Deeply knotted proteins, whose topologies may introduce substantial barriers to folding, thus represent an interesting test case for protein design. Here we report our attempts to design proteins with trefoil and pentafoil knotted topologies. We extended previously described algorithms for tandem repeat protein design in order to construct deeply knotted backbones and matching designed repeat sequences (N = 3 repeats for the trefoil and N = 5 for the pentafoil). We developed an approach for designing tandem repeat proteins that fold into a class of knotted topologies known as torus knots.

While kcTRP3c.1 and 3c.2 remained recalcitrant to crystallization, crystals of kcTRP3d.1, 3d.2, and 3d.3 grew readily, and their structures were solved via molecular replacement. kcTRP3d.1 and 3d.3 were phased with the original designed atomic coordinates of kcTRP3d as a molecular probe. Initial molecular replacement runs of kcTRP3d.2 also used kcTRP3d as a probe, however these failed to produce a solution. Only when kcTRP3d was truncated to a single helix-turn-helix equivalent to a single repeating domain (or motif, i.e. one-third of the trefoil) did we obtain a solution, which contained a single repeating subunit sitting on the 3-fold crystallographic axis. Since kcTRP3d.2 sits upon the 3-fold crystallographic axis, only a single repeating motif is present in the asymmetric unit (ASU). To obtain the full trefoil, crystallographic symmetry must be applied however this process averages the three repeating motifs of the trefoil into a single representation as well as averages out any remaining density from the flexible N-terminal affinity tag artifacts. This pseudo-symmetry and averaging are likely the cause of the higher-than-average R-values expected for a structure at this resolution. The kcTRP3d.2 construct crystallized in the intended space group (P213), with lattice dimensions and arrangement of molecules in the crystallographic unit cell that were similar to the lattice design model (55.35 Å vs 55.81 Å), but with differences in the lattice contacts corresponding to a register shift of one helical turn. The crystal structures of kcTRP3d.1–3 validated the accuracies of the designed molecular models and their intended deeply knotted topologies. Superposition of the structures to the original designed atomic coordinates of kcTRP3d produced all-atom rmsd values of 1.84 Å (kcTRP3d.1), 1.43 Å (kcTRP3d.2), and 1.90 Å (kcTRP3d.3).

> GSSMGSDEQRRELEEKIKWKLAELASKSEEERKEIKLRVIAYVLVQLEDLQKNLSDEQRRELEEKIKWKLAELASKSEEERKEIKLRVIAYVLVQLEDLQKNLSDEQRRELEEKIKWKLAELASKSEEERKEIKLRVIAYVLVQLEDLQKNLS>[4x]METVEEIKIADLRPNPYQPRKHFDDEALAELKESVLQHGILQPLIVRKSLKGYDIVAGERRFRAAKLAGLDTVPAIVRELSEALM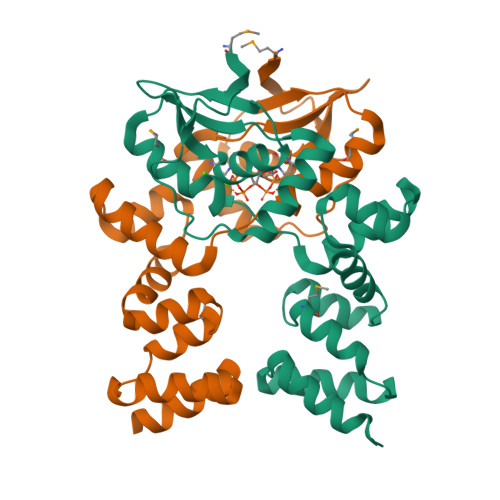REIALLENLQREDLSPLEEAQAYDSLLKHLDLTQEQLAKRLGKSRPHIANHLRLLTLPENIQQLIAEGTLSMGHGRTLLGLKNKNKLEPLVQKVIAEQLNVRQLEQLIQQLNQN>[2x]EKVIIEKAAGDAEAIAFDGRTYMEYHNAVTKSPDALDYPAEPSEKALQSN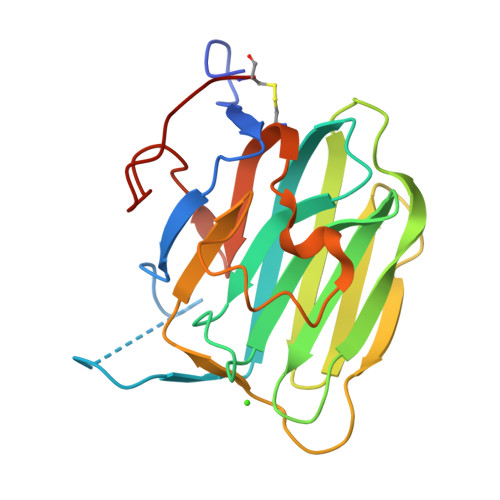HFELSIKTEATQGLILWSGKGLERSDYIALAIVDGFVQMMYDLGSKPVVLRSTVPINTNHWTHIKAYRVQREGSLQVGNEAPITGSSPLGATQLDTDGALWLGGMERLSVAHKLPKAYSTGFIGCIRDVIVDRQELHLVEDALNNPTILHCSAK> MTGGMKPPARKPRILNSDGSSNITRLGLEKRGWLDDHYHDLLTVSWPVFITLI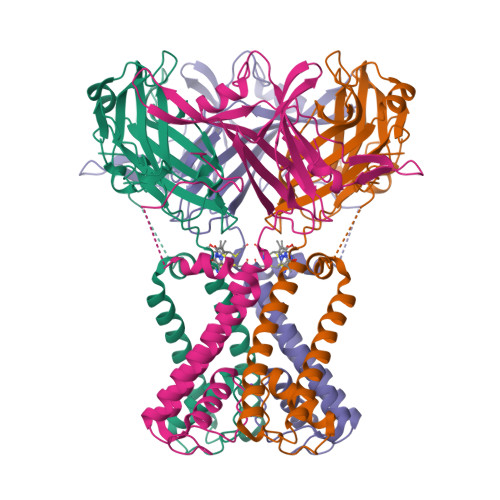TGLYLVTNALFALAYLAVGDVIENARPGSFTDAFFFSVQTMATIGYGKLIPIGPLANTLVTLEALVGMLGLAVAASLIYCRFCRPTAGVLFSSRMVISDFEGKPTLMMRLANLRIEQIIEADVHLVLVRSEISQEGMVFRRFHDLTLTRSRSPIFSLSWTVMHPIDHHSPIYGETDETLRNSHSEFLVLFTGHHEAFAQNVHARHAYSSDEIIWGGHFVDVFTTLPDGRRALDLGKFHEIAQHHHHHH Glutaryl-CoA dehydrogenase (GCDH) is an acyl-CoA dehydro­genase (ACDH) which catalyzes an intermediate step in the metabolic breakdown of lysine and tryptophan. Unlike other flavoproteins within this family, GCDH (EC 1.3.99.7) performs α,β-dehydrogenation as well as decarboxylation of its sub­strate glutaryl-CoA to yield the product crotonyl-CoA. Transfer of electrons from the glutaryl-CoA precursor to the electron-transfer flavoprotein is mediated by the cofactor flavin adenine dinucleotide (FAD) in both prokaryotic and eukaryotic electron-transport chains. Like other ACDHs, GCDH from B. pseudomallei (BpGCDH) exists as a homotetramer with tetrahedral symmetry and possesses an overall fold similar to that of the human enzyme.

Additional structures of BpGCDH resulting from this effort were obtained by soaking apo BpGCDH crystals in drops containing our Fragments of Life (FOL) ligand collection prior to data collection. All fragments identified by screening which bind BpGCDH occupy the pockets that bind the glutaryl and flavin moieties of the substrate and cofactor, respectively. In three of the four ligand-bound complexes fragment molecules occupy the binding site for the terminal glutamate of the glutaryl-coenzyme A substrate. The crystallographic water coordinated to the Arg97 side chain in the apo structure of BpGCDH remains in place when FOL544 is bound, but is displaced by FOL239 and FOL6421. In all three of these cases the Tyr373 side chain is rotated approximately 90° from its position in both the apo BpGCDH structure and the human ternary complex. This new position appears to facilitate ligand binding by providing a parallel aromatic surface that aligns with the heteroaromatic rings of all three fragments. However, a conserved backbone deviation is observed between the structure of apo BpGCDH and those of all four fragment-bound complexes in this same region. In all four fragment-bound structures Thr376 and His377 are flipped out of the α-helix observed in the apo state, partially occupying the binding pocket for the adenosine moiety of FAD. This perturbation results in a new orientation of the catalytic YEG motif. Thus, the binding of small metabolite-like ligands induces a conformation in apo crystals of BpGCDH that partially fills the FAD-binding site with protein residues.

>[4x]GPGSMAAATFHWDDPLLLDQQLADDERMVRDAAHAYAQGKLAPRVTEAFRHETTDAAIFREMGEIGLLGPTIPEQYGGPGLDYVSYGLIAREVERVDSGYRSMMSVQSSLVMVPIFEFGSDAQKEKYLPKLATGEWIGCFGLTEPNHGSDPGSMVTRARKVPGGYSLSGSKMWITNSPIADVFVVWAKLDEDGRDEIRGFILEKGCKGLSAPAIHGKVGLRASITGEIVLDEAFVPEENILPHVKGLRGPFTCLNSARYGIAWGALGAAESCWHIARQYVLDRKQFGRPLAANQLIQKKLADMQTEITLGLQGVLRLGRMKDEGTAAVEITSIMKRNSCGKALDIARLARDMLGGNGISDEFGVARHLVNLEVVNTYEGTHDIHALILGRAQTGIQAFF(Z)-hexadec-9-enal | C16 H30 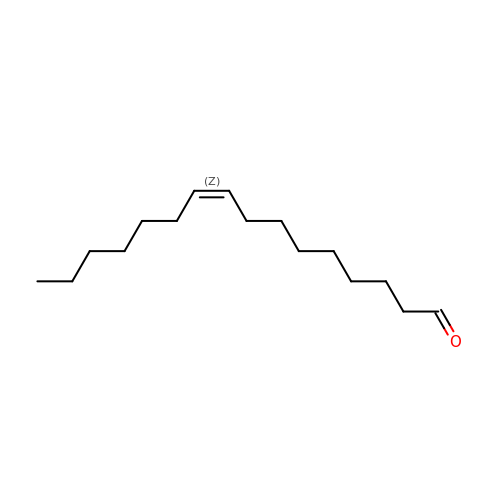O | QFPVVMKZTVQDTL-FPLPWBNLSA-N>[2x]MKPATYNTEAFDEWIRSRFVELNSQLEQLYYQQTDRANVQEVGTELKHTLESEGRELVKALLDEGNTDEGFDSAFDLLGNVGLYMAACRRHEITEPTRETTSPLLEASALAMHIGAS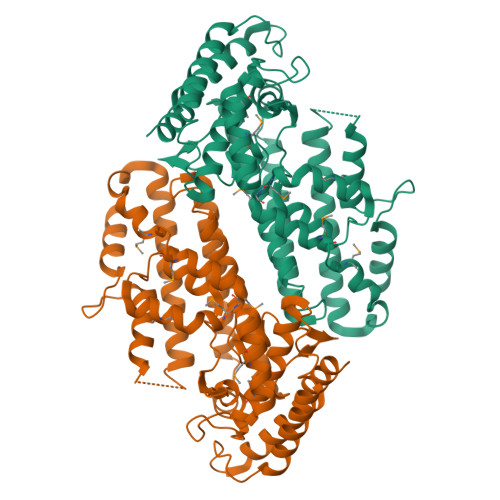IGVTPRFATAHLTTHNRAHNGIYKRFTDLPDEKLFVDYNTKGILAYKRASDALLKIQPLGISHPISHDLLRVTKQALQDVIESNQQLFNRLDTDRFFYCVRPYYKPYRVGSVVYRGANAGDFAGINVIDLTLGLCFANEASYSQMLVDKFLYMMPEDQQILRECMRRPNLMDDFLQAKGCIHQDWYQENLKLFIEVCELHGQTAIQHHNELVTKYIAEPSVSMEQQHLAKVTASGPPLHVLLASLERLRDRRAAVLRDDIRTRYYDLKKLKDSLRLEAAAHHHHHH>[2x]MAEAASCARKGTKYAEGTQPFTVLIEGNIGSGKTTYLNHFEKYKNDICLLTEPVEKWRNVNGVNLLELMYKDPKKWAMP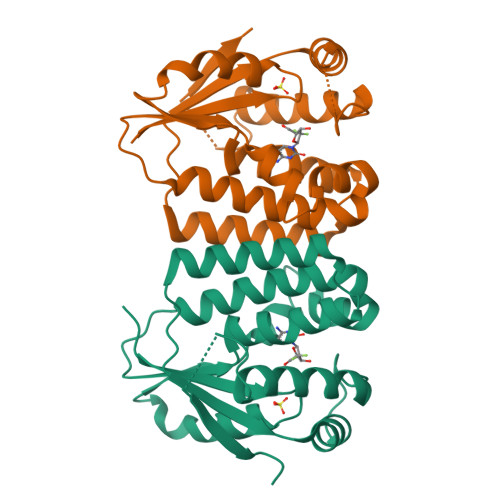FQSYVTLTMLQSHTAPTNKKLKIMERSIFSARYCFVENMRRNGSLEQGMYNTLEEWYKFIEESIHVQADLIIYLRTSPEVAYERIRQRARSEESCVPLKYLQELHELHEDWLIHQRRPQSCKVLVLDADLNLENIGTEYQRSESSIFDAIS>[6x]MKKLTIGLIGNPNSGKTTLFNQLTGSRQRVGNWAGVTVERKEGQFSTTDHQVTLVDLPGTYSLTTISSQTSLDEQIACHYILSGDADLLINVVDASNLERNLYLTLQLLELGIPCIVALNMLDIAEKQNIRIEIDALSARLGCPVIPLVSARGR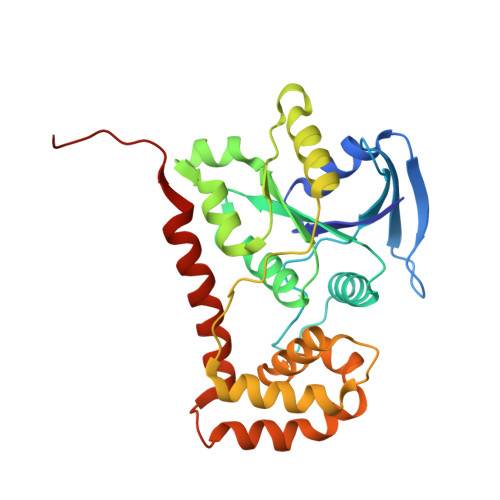GIEALKLAIDRYKANENVELVHYAQPLLNEADSLAKVMPSDIPLKQRRWLGLQMLEGDIYSRAYAGEASQHLDAALARLRNEMDDPALHIADARYQCIAAICDVVSNTLTAEPSRF>MKYVVVSGGVISGIGKGVLASSTGMLMKTLGLKVTSIKIDPYMNIDAGTMSPLEHGECFVLDDGGETDLDLGNYERYLGVTLTKDHNITTGKIYSHVIAKERKGDYLGKTVQIVPHLTNAIQDWIERVAKIPVDD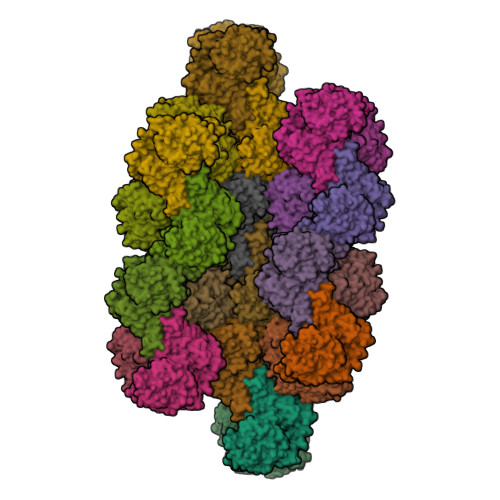TGMEPDVCIIELGGTVGDIESAPFVEALRQFQFKVGKENFALIHVSLVPVIHGEQKTKPTQAAIKGLRSLGLVPDMIACRCSETLDKPTIDKIAMFCHVGPEQVVNVHDVNSTYHVPLLLLEQKMIDYLHARLKLDEISLTEEEELLSKWKATTGNFDETVKIALVGKYTNLKDSYLSVIKALEHSSMKCRRKLDIKWVEATDLEPEAQESNKTKFHEAWNMVSTADGILIPGGFGVRGTEGMVLAARWARENHIPFLGVCLGLQIATIEFTRSVLGRKDSHSAEFYPDIDEKNHVVVFMMRLGLRPTFFQNETEWSQIKKLYGDVSEVHERHRHRYEINPKMVDELENNGLIFVGKDDTGKRCEILELKNHPYYIATQYHPEYTSKVLDPSKPFLGLVAASAGILQDVIEGKYDLEA[28x]> GDITHMEKLGD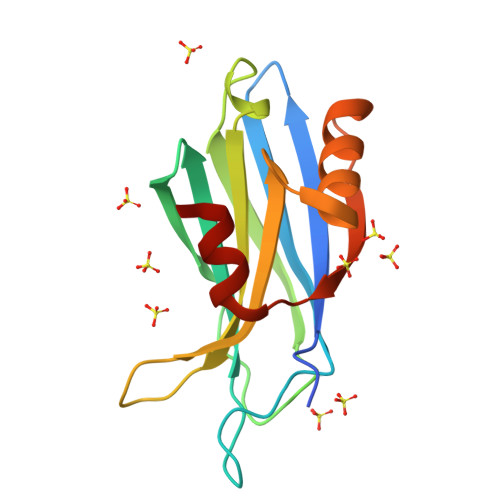ICFSLRYVPTAGKLTVVILEAKNLKKMDVGGLSDPYVKIHLMQNGKRLKKKKTTIKKNTLNPYYNESFSFEVPFEQIQKVQVVVTVLDYDKTGKNDAIGKVFVGYNSTGAELRHWSDMLANPRRPIAQWHTLQVEEEVDAMLAVKK> GSHMLKDSLRPKLSEEQQHIIAILLDAHHKTYDPTYADFRDFRPPVRMDGSTGSVTLDLSPLSMLPHLADLVSYSIQKVIGFAKMIPGFRDLTSDDQIVLLKSSAIEVIMLRSNQSFTMDDMSWDCGSQDYKYDVTDVSKAGHTLELIEPLIKFQVGLKKLNLHEEEHVLLMAICIVSPDRPGVQDAKLVEAIQDRLSNTLQTYIRCRHPPPGSHQLYAKMIQKLADLRSLNEEHSKQYRSLSFQPEN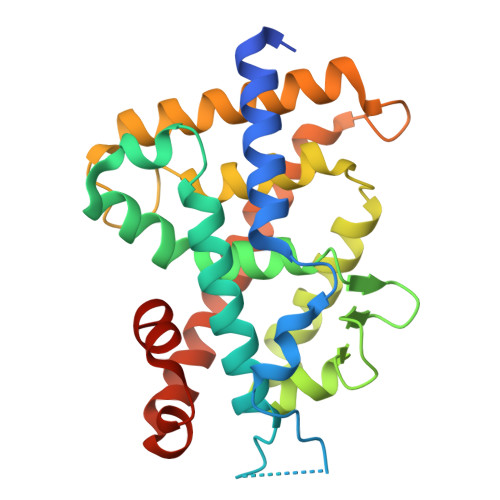SMKLTPLVLEVFGNEIS>MRGKVYLVGAGFGGPEHLTLKALRVLEVAEVVLHDRLVHPGVLALAKGELVPVGKEGYGGKTPQEAITARLIALAREGRVVARLKGGDPMVFGRGGEEALALRRAGIPFEVVPGVTSAVGALSALGLPLTHRGLARSFAVATGHDPALPLPRADTLVLLMPLHTLGGLKERLLERFPPETPLALLARVGWPGEAVRLG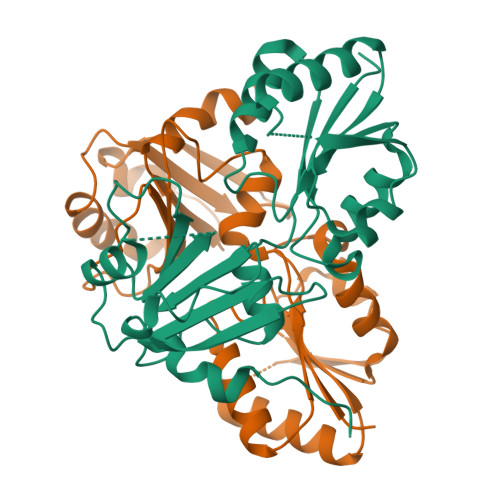RVEDLPGLGEGLPSPALLVVGKVVGLYGELLPKDHGL[2x]>STNDNIKDLLDWYSSGSDTFTNSEVLDNSLGSMRIKNTDGSISLIIFPSPYYSPAFTKGEKVDLNTKRTKKSQHTSEGTYIHFQISGVTNTEKLPTPIELPLKVKVHGKDSPLKYWPKFDKKQLAISTLDFEIRHALTQIHGLYRSSDKTGGYWKITMNDGSTYQSDLSKKFEYNTEKPPINIDEIKTIEA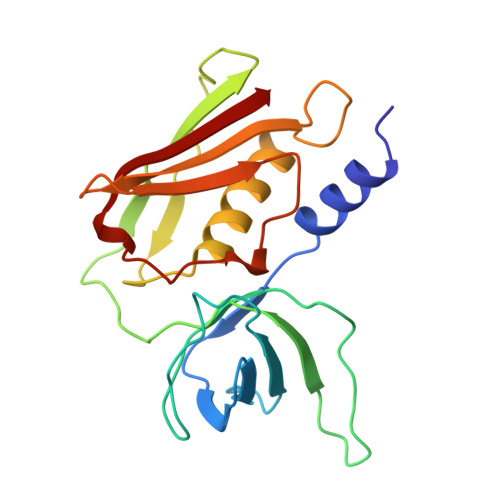EIN[4x]>SNAFLDYGLSEADPDVHAIINKEKDRQFRSLELIASENFTSKAVMEAVGSCLTNKYSEGLPGKRYYGGNEHIDELEILCQQRALAAFHLDGDKWGVNVQPLSGSPANFAVYTAILKPHDRIMGLDLPHGGHLSHGFMTAKRRVSGTSIYFESMPYRLDESTGVIDYDMLEKTAALFRPKLIIAGASAYPRDIDYARFRKIADSVGAFLMMDMAHVSGLIAASVLADPFEFVDIVTTTTHKSLRGPRGGMIFFKKDAVHGVDLESAINNAVFPGLQGGPHNHTIGGLAVCLKYAQSPDFKNYQNQVVANCRALANRLVEHEYKLVSGGSDNHLVLVDLRPSGIDGARVEKILDMASITLNKNSVPGDKSALVPGGIRIGSPAMTTRGLGEKEFELIADLIHEGVRISLEAKSLVSGTKVQDFLNFVLAPEFPLGDKVSNLRRKVEALATQYPIPGV[2x]

SHMTs are α-class pyridoxal 5′-phosphate (PLP)-dependent enzymes which transfer hydroxymethyl of Ser to – typically polyglutamylated (polyGlu) – tetrahydrofolate (H4PteGlun), producing Gly and 5,10-CH2-H4PteGlun. Here we report crystal structures of a chloroplastic SHMT enzyme from the model legume plant, Medicago truncatula (Mt), which similarly to At has seven SHMT isoforms. MtSHMT3 is a member of the α-class of PLP enzymes, and its overall fold is typical for this family. A subunit of MtSHMT3 can be subdivided into three regions: N-terminal arm, large domain, and small domain, consistently with other SHMTs.

The crystal structure of MtSHMT3 (residues 82–533), which is the first structure of a plant SHMT, was solved using the recently developed phasing method that utilizes selenourea soaking. MtSHMT3 crystals soaked with selenourea served to solve the structure experimentally by single anomalous dispersion (SAD) phasing. Based on the anomalous difference maps, at least twenty selenourea molecules were bound to the protein, often via extensive networks of hydrogen bonds.>[2x]EPRAEDGHAHDYVNEAADASGHPRYQEGQLCENCAFWGEAVQDGWGRCTHPDF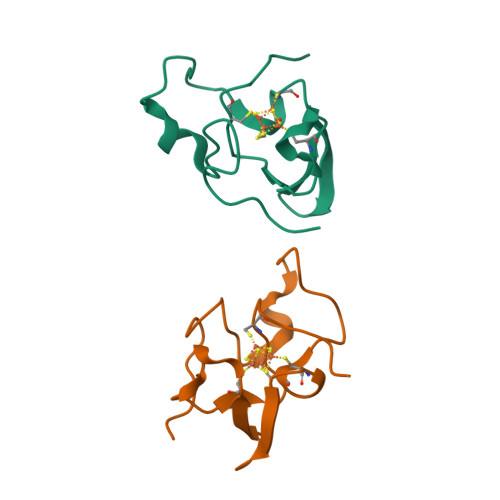DEVLVKAEGWCSVYAPASS> QRPEPTPEEWDLIHIATEAHRSTNAQGSHWKQRRKFLPDDIGQSPIVSMPDGDKVDLEAFSEFTKIITPAITRVVDFAKKLPMFSELPCEDQIILLKGCCMEIMSLRAAVRYDPESDTLTLSGEMAVKREQLKNGGLGVVSDAIFELGKSLSAFNLDDTEVALLQAVLLMSTDRSGLLCVDKIEKSQEAYLLAFEHYVNHRKHNIPHFWPKLLMKVTDLRMIGACHASRFLHMKVE

The physiological effects of thyroid hormones (TH; T4, thyroxine; T3, triiodothyronine) are mediated by their canonical action via nuclear thyroid hormone receptors (TRs; TRα and TRβ) with differing tissue distributions, which regulate the transcription of target genes in a ligand-dependent manner. Unliganded TRs recruit a multiprotein complex which contains corepressor (CoR; e.g., nuclear receptor corepressor [NCoR] or silencing mediator of retinoic acid and thyroid hormone receptor [SMRT]) and histone deacetylase (HDAC) to inhibit target gene transcription. Receptor occupancy by a ligand (T3) promotes the dissociation of this corepressor complex with the relief of transcriptional repression and mediates the recruitment of a protein complex containing coactivators (e.g., NCoA-1/SRC-1, NCoA-2/GRIP-1, and NCoA-3/ACTR) with chromatin-remodeling activity, inducing the transcription of target genes. Mutations in thyroid hormone receptor α (TRα), a ligand-inducible transcription factor, cause resistance to thyroid hormone α (RTHα).

Accordingly, to model the human TRα mutants, we crystallized an artificial mutant receptor (P393GX) which was truncated at the carboxy terminus of helix 11. Importantly, the P393GX TRα shows similar molecular behavior to the human TRα mutants. Small crystals of P393GX in complex with T3 were obtained which diffracted to 3.0 Å. The structure contains one P393GX molecule (amino acids 156 to 393) and one T3 molecule in the asymmetric unit. However, despite having the potential to form a complete helix 11 (aa 363 to 393), in the P393GX mutant TRα this helix terminates at Ala 379, with the peptide backbone turning at this point to form an extended coil which runs antiparallel to the adjacent helix 5 toward the corepressor-binding site. The T3 ligand could be placed unambiguously in the hydrophobic cavity of P393GX TRα LBD and binds very similarly to its occupancy of wild-type receptor LBD. However, T3 interactions with Met 388 and Phe 401 are lost and the orientation of His 381 is altered. Arg 384 makes a new interaction with the ligand in the P393GX LBD, donating a hydrogen bond to the 4′ hydroxyl of the outer ring of T3. Interestingly, the lack of the carboxy-terminal end of helix 11 and the joining of the loop to helix 12 creates space for residues amino-terminal to helix 3 to form a short anti-parallel β-sheet, which is not present in the wild-type receptor. Remarkably, given that so much of the receptor carboxy terminus is missing, the ligand binding cavity in P393GX mutant TRα is almost completely enclosed due to the rearrangement of the carboxy-terminal portion of helix 11.> VETISFSFSEFEPGNDNLTLQGASLITQSGVLQLTKINQNGMPAWDSTGRTLYAKPVHIWDMTTGTVASFETRFSFSIEQPYTRPLPADGLVFFMGPTKSKPAQGGGYLGIFNNSKQDNSYQTLGVEFDTFSNQ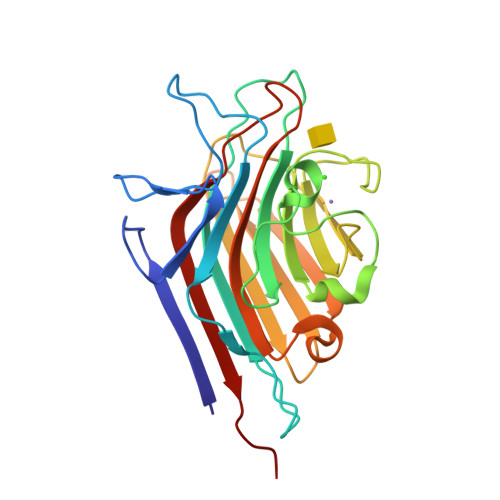WDPPQVPHIGIDVNSIRSIKTQPFQLDNGQVANVVIKYDASSKILHAVLVYPSSGAIYTIAEIVDVKQVLPEWVDVGLSGATGAQRDAAETHDVYSWSFQASLPETND> GLPVINTPGSNQFLTSDDFQSPSAMPQFDVTPELNIPGEVQNLMEIAEVDSVVPVNNVAGNLETMDIYRIPVQSGNHQSSQVFGFQVQPGLDGVFKHTLLGEILNYYAHWSGSIKLTFVFCGSAMATGKFLLAYAPPGANAPKSRKDAMLGTHIIWDVGLQSSCVLCIPWISQTHYRLVQ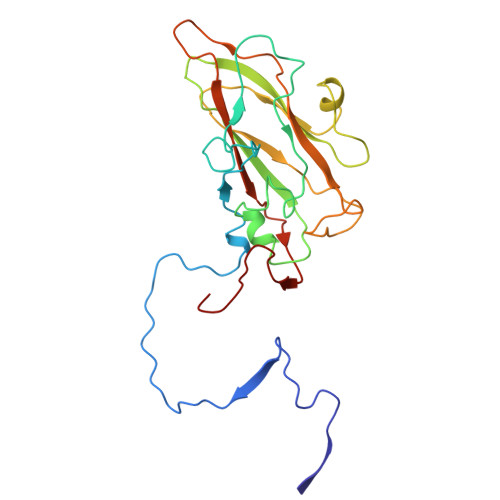QDEYTSAGNVTCWYQTGIVVPAGTPTSCSIMCFVSACNDFSVRLLKDTPFIQQAALLQ>[4x]MVEKFVGTWKIADSHNFGEYLKAIGAPKELSDGGDATTPTLYISQKDGDKMTVKIEAGPPTFLD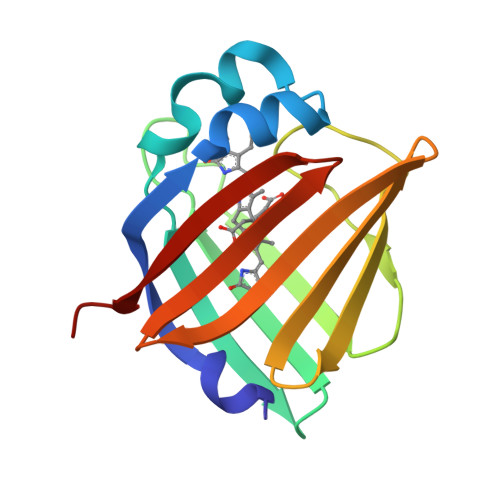TQVKFKLGEEFDEFPSDRRKGVKSVVNLVGEKLVYVQKWDGKETTYVREIKDGKLVVTLTMGDVVAVRSYRRATE>[2x]GMAKKTLILYYSWSGETKKMAEKIN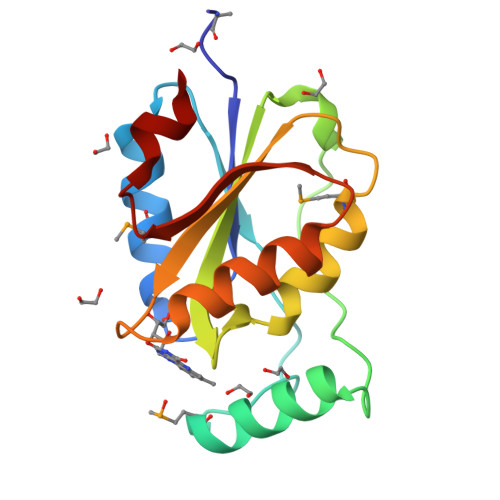SEIKDSELKEVKVSEGTFDADMYKTSDIALDQIQGNKDFPEIQLDNIDYNNYDLILIGSPVWSGYPATPIKTLLDQMKNYRGEVASFFTSAGTNHKAYVSHFNEWADGLNVIGVARDDSEVDKWSK>[2x]UUGCG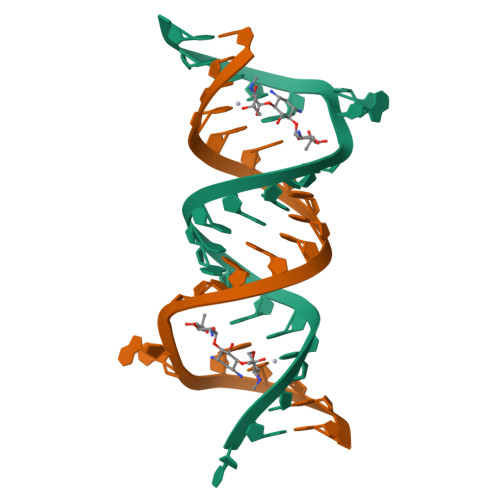UCGCGUCGACGAAGUCGC> MATVEPETTPTPNPPTTEEEKTESNQEVANPEHYIKHPLQNRWALWFFKNDKSKTWQANLRLISKFDTVEDFWALYNHIQLSSNLMPGCDYSLFKDGIEPMWEDEKNKRGGRWLITLNKQQRRSDLDRFWLETLLCLIGESFDDYSDDVCGAVVNVRAKGDKIAIWTTECENREAVTHIGRVYKERLGLPPKIVIGYQSHADTATKSGSTTKNRFVV;> KKRYDREFLLGFQF

Initially, the 40S ribosomal subunit associates with Met-tRNAi and a group of initiation factors, including eIF1, eIF1A, eIF2, eIF3, and eIF5 to form the 43S pre-initiation complex. This complex is then recruited to the 5′-end of capped mRNA by another complex of factors (known as eIF4F) consisting of eIF4E, eIF4G, and eIF4A. eIF4E is an indispensable element for cap-dependent translation initiation and plays a major role in recognition of the mRNA cap structure (m7GpppN, where N is any nucleotide). Under resting conditions, eIF4E is kept in an inactive form bound to 4E-binding proteins (4E-BPs); once the latter have been phosphorylated through the PI3K-AKT-mTOR signalling pathway, eIF4E is released and can associate with eIF4G to launch translation. eIF4E is overexpressed in numerous human tumours, and it contributes to transformation, tumourigenesis, and progression of cancers. eIF4E overexpression facilitates translation of weak and highly structured mRNAs that typically encode proteins involved in cancer pathology, such as proto-oncoproteins (e.g. cyclin D1, ornithine decarboxylase), angiogenesis factors (e.g. FGF-2, VEGF), and factors related to tumour invasiveness, such as MMP-9, due to the ability of eIF4E to stimulate eIF4A. All complex structures showed the characteristic cupped hand structure of eIF4E with the ligands occupying the cap-binding site.

The positively charged N7-methyl guanine system forms the characteristic cation-π interaction as expected. Fig. 7b shows compound 4f bound to the cap-binding site of eIF4E. The guanine group is located in its normal binding position, stacking with the side-chain of W56. As predicted, the squaramide occupies the α-phosphate position, making interactions with the side-chain of R157. The chloro substituent of the N7-benzyl group causes a rotation of approximately 90° in relation to other N7-benzyl substituted cap analogues. In turn, to accommodate the extra space required by the chloro group, the side chain of W102 is re-oriented away from making the usual cation-π stacking interaction to a position similar to that seen with 7a in the presence of sulfate (compare Fig. 6). Furthermore, substitution of the phenyl group with small and electronically neutral groups (3-Me, 4c; 3-Cl, 4f) retained the modest activity of 4a and 4b, whereas introduction of larger and more polar substituents reduced or abolished activity. However, our structures highlight the flexibility of the m7G-binding pocket, especially residue W102 that forms part of the cation-π interaction characteristic of cap-recognition by eIF4E.> MAEGNTLISVDYEIFGKVQGVFFRKHTQAEGKKLGLVGWVQNTDRGTV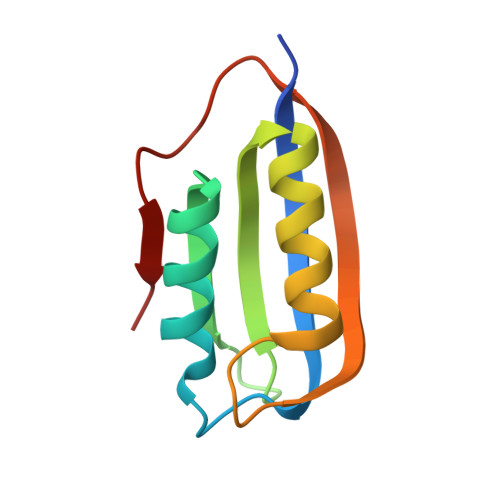QGQLQGPISKVRHMQEWLETRGSPKSHIDKANFNNEKVILKLDYSDFQIVA>[5x]GSHMDFEIEVMNYSIEEFREFKTTDVESVLPFRDSSTPTWINITGIHRTDVVQRVGEFFGIHPLVLEDILNVHQRPKVEFFENYVFIVLKMFTYDKNLHELESEQVSLILTKNCVLMFQEKIGDVFDPVRERIRYNRGIIRKKRADYLLYSLIDALVDDYFVLLEKIDDEIDVLEEEVLERPEKETVQRTHQLKRNLVELAATIWPLREVLSSLYRDVP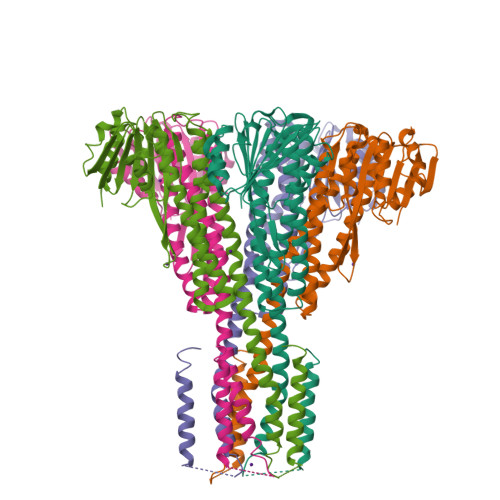PLIEKETVPYFRDVYDHTIQIADTVETFRDIVSGLLDVYLSSVSNKTNEVMKVLTIIATIFMPLTFIAGIYGMNFEYMPELRWKWGYPVVLAVMGVIAVIMVVYFKKKKWL> GRSRLLEDFRNNRFPNLQLRDLIGHIVEFSQDQHGSRFIQQKLERATPAERQMVFNEILQAAYQLMTDVFGNYVIQKFFEFGSLDQKLALATRIRGHVLPLALQMYGCRVIQ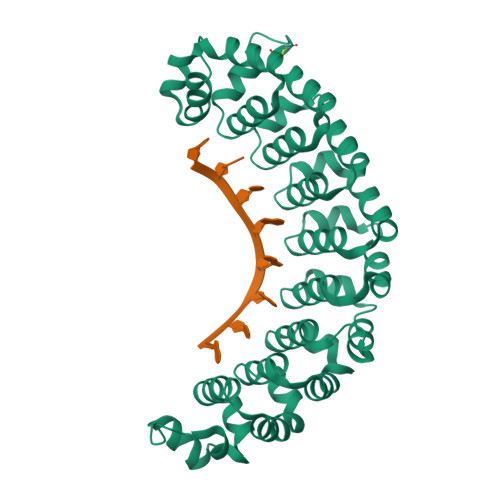KALESISSDQQVISEMVKELDGHVLKCVKDQNGNHVVQKCIECVQPQSLQFIIDAFKGQVFVLSTHPYGCRVIQRILEHCTAEQTLPILEELHQHTEQLVQDQYGNYVIQHVLEHGRPEDKSKIVSEIRGKVLALSQHKFASNVVEKCVTHASRAERALLIDEVCCQNDGPHSALYTMMKDQYANYVVQKMIDMAEPAQRKIIMHKIRPHITTLRKYTYGKHILAKLEKYYLKNSPDLG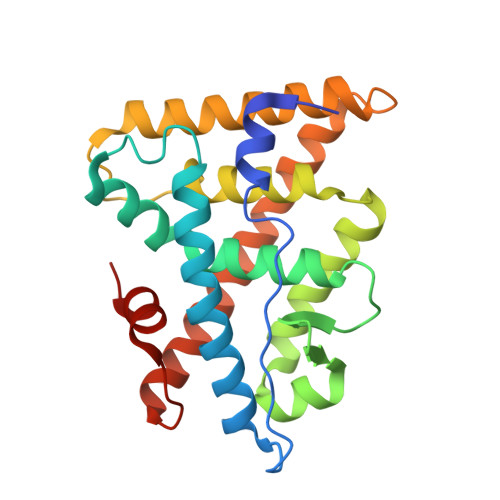> PAKKPYNKIVSHLLVAEPEKIYAMPDPTVPDSDIKALTTLCDLADRELVVIIGWAKHIPGFSTLSLADQMSLLQSAWMEILILGVVYRSLSFEDELVYADDYIMDEDQSKLAGLLDLNNAILQLVKKYKSMKLEKEEFVTLKAIALANSDSMHIEDVEAVQKLQDVLHEALQDYEAGQHMEDPRRAGKMLMTLPLLRQTSTKAVQHFYNIKLEGKVPMHKLFLEMLEAKV>MAGLLKESMRIKMYMEGTVNGHYFKCEGEGDGNPFAGTQSMRIHVTEGAPLPFAFDILAPCCEYGSRTFVHHTAEIPDFFKQSFPEGFTWERTTTYEDGGILTAHQDTSLEGNCLIYKVKVHGTNFPADGPVMKNKSGGWEP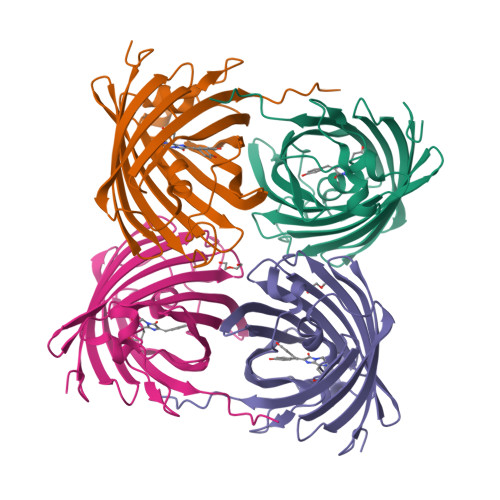STEVVYPENGVLCGRNVMALKVGDRHLICHHYTSYRSKKAVRALTMPGFHFTDIRLQMLRKKKDEYFELYEASVARYSDLPEKAN[4x]> MSASTLSRLLPAGSLAWGLPGVLLRSASLLVHHQPCAPSTSGRVQESQLQWSCYYATSHGTGAPKAASTQSSSTTSAASAAASATSAARPAAVSSE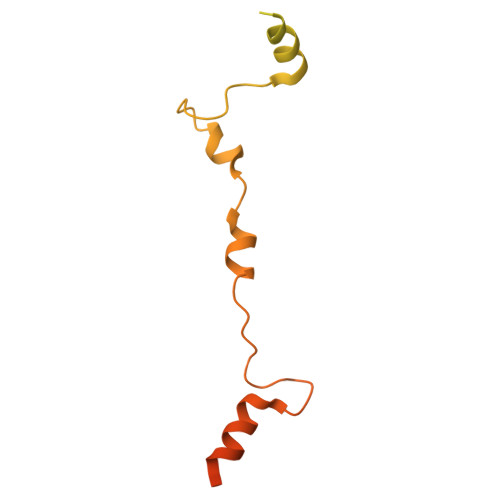AGGDGASSAPFYAGLAARYPDPDTVPDHVMHRLRNTLFGRAVRPRETTGRRALARPLQGKALTDWYWMPPNESPGFHSEEDEYELRRALNRRHTKEAEAEAADTGADKKKKRK> 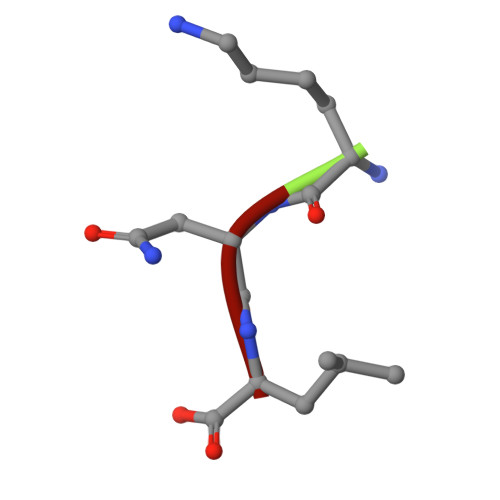KNL2-(2-{4-[(6-aminopyridin-3-yl)sulfonyl]piperazin-1-yl}-3,3'-bipyridin-5-yl)-1,1,1,3,3,3-hexafluoropropan-2-ol | C22 H20 F6 N6 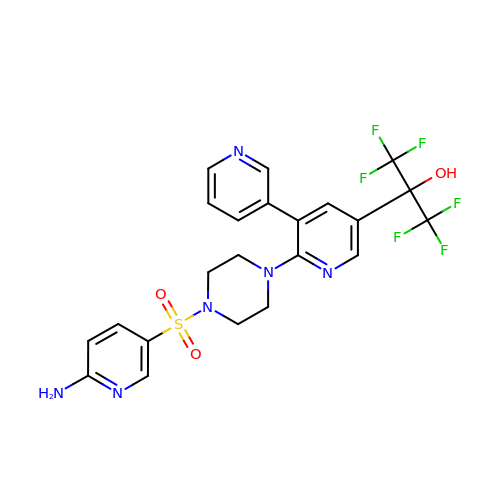O3 S | WSCXEOSPTMGMGQ-UHFFFAOYSA-N>MNQNLLVTKRDGSTERINLDKIHRVLDWAAEGLHNVSISQVELRSHIQFYDGIKTSDIHETIIKAAADLISRDAPDYQYLAARLAIFHLRKKAYGQFEPPALYDHVVKMVEMGKYDNHLLEDYTEEEFKQMDTFIDHDRDMTFSYAAVKQLEGKYLVQNRVTGEIYESAQFLYILVAACLFSNYPRETRLQYVKRFYDAVSTFKISLPTPIMSGVRTPTRQFSSCVLIECGDSLDSINATSSAIVKYVSQRAGIGINAGRIRALGSPIRGGEAFHTGCIPFYKHFQTAVKSCSQGGVRGGAATLFYPMWHLEVESLLVLKNNRGVEGNRVRHMDYGVQINKLMYTRLLKGEDITLFSPSDVPGLYDAFFADQEEFERLYTKYEKDDSIRKQRVKAVELFSLMMQERASTGRIYIQNVDHCNTHSPFDPAIAPVRQSNLCLEIALPTKPLNDVNDENGEIALCTLSAFNLGAINNLDELEELAILAVRALDALLDYQDYPIPAAKRGAMGRRTLGIGVINFAYYLAKHGKRYSDGSANNLTHKTFEAIQYYLLKASNELAKEQGACPWFNETTYAKGILPIDTYKKDLDTIANEPLHYDWEALRESIKTHGLRNSTLSALMPSETSSQISNATNGIEPPRGYVSIKASKDGILRQVVPDYEHLHDAYELLWEMPGNDGYLQLVGIMQKFIDQSISANTNYDPSRFPSGKVPMQQLLKDLLTAYKFGVKTLYYQNTRDGAEDAQDDLVPSIQDDGCESGACKI[4x];>[4x]AYTTFSQTKNDQLKEPMFFGQPVNVARYDQQKYDIFEKLIEKQLSFFWRPEEVDVSRDRIDYQALPEHEKHIFISNLKYQTLLDSIQGRSPNVALLPLISIPELETWVETWAFSETIHSRSYTHIIRNIVNDPSVVFDDIVTNEQIQKRAEGISSYYDELIEMTSYWHLLGEGTHTVNGKTVTVSLRELKKKLYLCLMSVNALEAIRFYVSFACSFAFAERELMEGNAKIIRLIARDEALHLTGTQHMLNLLRSGADDPEMAEIAEECKQECYDLFVQAAQQEKDWADYLFRDGSMIGLNKDILCQYVEYITNIRMQAVGLDLPFQTRSNPIPWINTWLVSDNVQVAPQEVEVSSYLVGQIDSEVDTDDLSNFQL

Deoxyribonucleotides, the building blocks for DNA biosynthesis, are produced in the cell from ribonucleotide precursors by ribonucleotide reductase (RNR). The best characterized of all RNRs is the class Ia enzyme from Escherichia coli that employs a di-iron-tyrosyl-radical cofactor to initiate chemistry and requires two dimeric protein subunits for enzymatic activity. As a central controller of nucleotide metabolism, RNR uses multiple allosteric mechanisms to maintain the balanced deoxyribonucleoside triphosphate (dNTP) pools that are required for accurate DNA replication. Briefly, the binding of (d)NTP effectors to an allosteric specificity site in α2 influences the preference of RNR for its four nucleoside diphosphate (NDP) substrates.

We have utilized an α4β4 crystal form of the E. coli class Ia RNR (right) to obtain structures of all four substrate/specificity effector pairs (CDP/dATP, UDP/dATP, ADP/dGTP or GDP/TTP) bound to the α2 subunit. Each model consists of two α2 dimers, two β2 dimers, and activity effector dATP in all four allosteric activity sites. Whereas high levels of dATP inhibit class Ia RNR, at lower levels, dATP promotes CDP or UDP reduction. The remaining interactions with loop 2 are distinct for each substrate/effector pair. dATP, which preferentially increases RNR activity for CDP and UDP substrates, makes two hydrogen bonds with loop 2. The backbone amide and carbonyl of Ser293 are in position to hydrogen bond to N1 and N6, respectively, of the adenine base of dATP. These hydrogen bonds hold Ser293 in place and position the adjacent Gln294 in to a conformation that points into the substrate-binding site. In this conformation, Gln294 can form a hydrogen bond with O2 of CDP or UDP. There is no difference in substrate positioning between CDP and UDP, as the unique positions of the pyrimidine ring (N2 and N4/O4) are not involved in any contacts with the protein. Briefly, dATP, which enhances reduction of CDP/UDP, makes specific contacts with Ser293, orienting Gln294 toward the active site and stabilizing the binding of both CDP and UDP. The lack of discrimination between CDP and UDP substrates by RNR is not problematic for the cell as cytidine deaminase provides another level of control for dCTP/TTP ratios.(2S)-2-{[(1-chloro-4-hydroxyisoquinolin-3-yl)carbonyl]amino}propanoic 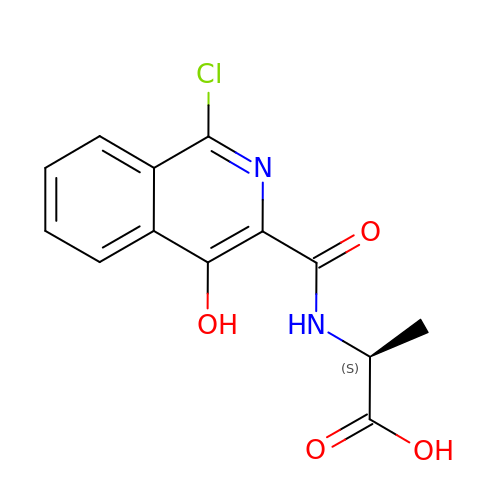acid | C13 H11 Cl N2 O4 | QJWFWOUODUTVCE-LURJTMIESA-M Sabinene 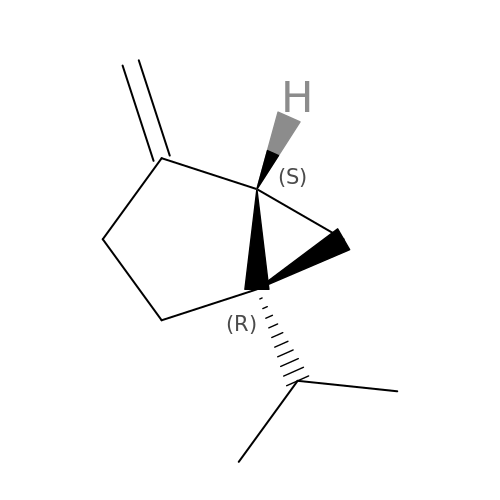| C10 H16 | NDVASEGYNIMXJL-UWVGGRQHSA-N> MTSKKRARDEEAQSGGSEAETKPAPVKKA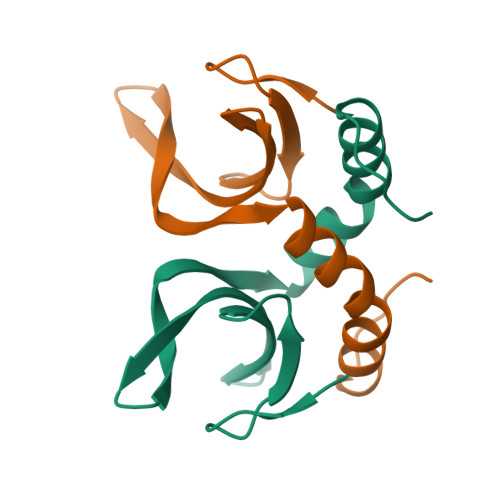KSKASNPGGSQVDAEGNPFWEISDKRRVGISQFKKMDFINIREYYEAGGEMKPGKKGIGLTVDQYTAFLKAIPAINAELRSRGHDITDDSDGGGAPVVAKPEGNAKKSTKKQEKKANIEATSDEGSGSD>[4x]MRFTILSVLAFSLPLVLAETPAPSCPVTNVTTPQLDPITQAYADAISSRPSLFAFPLPEIRDGYQSNVSDPSTEFTTKILSLPVGPTGNVTAYLYKPVSGEREKGKDLLPVIAYFHGGGWVFGGPKSYRGLITNLIRESGAAVFFVDYTLTPKVAYPVPNEQCYAAVQWLLEHGEKLGVDPTNMGFGGDSAGGELSSSVSLLSIKRKTPLPKFQVLIYPATDLACESATFKEFPNGPGLTTDEIRFAASLFTPDPKSRLEDVASPGRASDEDLAKFPETLIVVAEVDPIRQQGEDFGRRLQKLGVRAAIIRVLGTIHGFASIDVLSEAPGAKATIELIGYKFKKALH

We present here the results of a detailed functional characterization and 3D structure analysis of these three T. melanosporum enzymes, designated as TmelEST 1, 2 and 3, which are shown to be non-lypolitic HSL carboxylesterases closely resembling archaeal and endosymbiotic soil bacteria esterases. The 3D structure of TmelEST2 shows an α/β-hydrolase-fold with well discernible cap and catalytic domains. The latter contains the core region with the catalytic Ser-His-Asp triad, while the less conserved and more dynamic cap domain controls access to the active site and thus likely determines substrate selectivity. The active site of TmelEST2 comprises the Ser190 nucleophile located within the conserved Gly-X-Ser-X-Gly motif, the proton carrier His317 (β7) and the other charge-relay network residue Asp287 (β8).

As expected for hydrolytic enzymes bearing a catalytic serine residue, TmelESTs were all irreversibly inhibited by phenylmethylsulfonyl fluoride (PMSF, 2 mM; data not shown). Additional details of the active site architecture were revealed by parallel analysis of a TmelEST2-PMSF structure, showing the sulfonyl fluoride group of the inhibitor covalently bound to the Oγ of Ser190 in all four monomers. In this structure, the Oα of the PMSF sulfonyl group is hydrogen-bonded to the NH groups of Gly119 and Ala191, while the benzyl group points toward Ala247 within the hydrophobic substrate tunnel. The structures of the catalytic domain, including the active site and the oxyanion hole, are, instead, essentially superimposable among the three enzymes and remain essentially unaltered upon PMSF incorporation, at least in the case of TmelEST2. The different kinetic properties of the Tuber carboxylesterases are thus likely to be ascribed to other regions of the protein and/or to subtle differences in active site flexibility or protein dynamics.(1-{2-[4-(diphenylmethyl)piperazin-1-yl]-2-oxoethyl}cyclopentyl)acetic 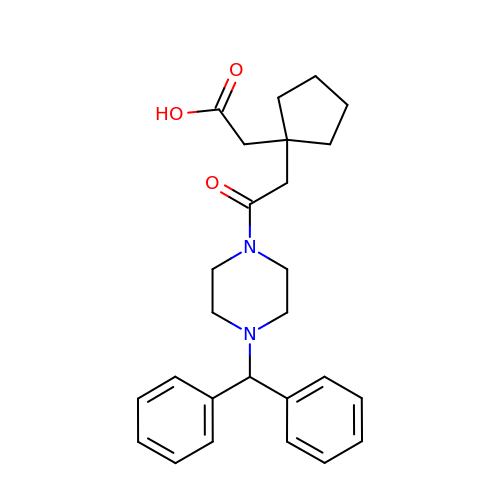acid | C26 H32 N2 O3 | GLJDWAQYHLAMPV-UHFFFAOYSA-N>MPVSNAQLTQMFEHVLKLSRVDETQSVAVLKSHYSDPRTVNAAMEAAQRLKAKVYAVELPAFNHPTAMGNDMTAYCGDTALTGNLAAQRALEAADLVVDTMMLLHSPEQEQILKTGTRILLAVEPPEVLARMLPTEDDKRRVLAAETLLKQARSLHVRSKAGSDFHAPLGQYPAVTEYGYADEPGRWDHWPSGFLFT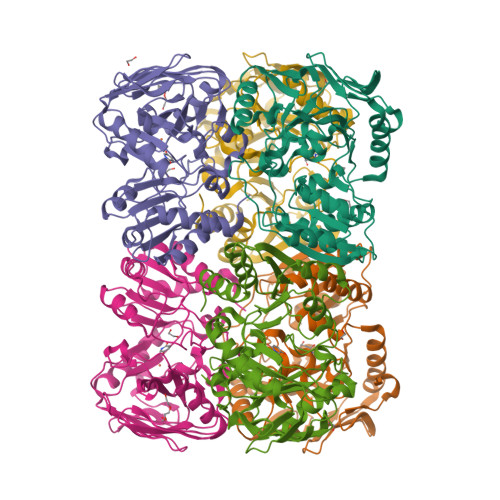WPNEDSAEGTLVLDVGDIILPFKNYCRERITLEIEKGFITGIHGGFEAEYLRDYMKYFNDPEVYGISHIGWGLQPRAQWTAMGLHDRNDGMCMDARAFYGNFLFSTGPNTEVGGKRKTPCHLDIPLRNCDIYLDDKAVVLAGDVVAPEESRARKLAAALEHHHHHH[6x]(1R, 2S)-CIS 1,2 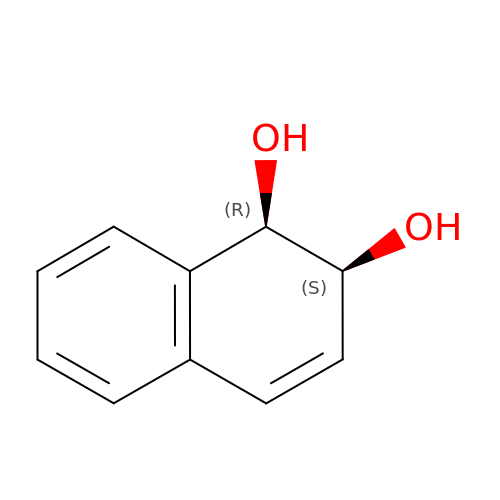DIHYDROXY-1,2-DIHYDRONAPHTHALENE | C10 H10 O2 | QPUHWUSUBHNZCG-VHSXEESVSA-N> MEFFGESWKKHLSGEFGKPYFIKLMGFVAEERKHYTVYPPPHQVFTWTQMCDIKDVKVVILGQDPYHGPNQAHGLCFSVQRPVPPPPSLENIYKELSTDIEGFVHPGHGDLSGWAKQGVLLLNAVLTVRAHQANSHKERGWE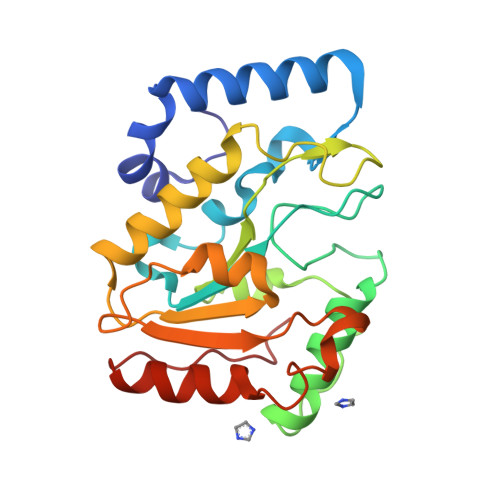QFTDAVVSWLNQNSNGLVFLLWGSYAQKKGSAIDRKRHHVLQTAHPSPLSVYRGFFGCRHFSKTNELLQKSGKKPIDWREL> KTRY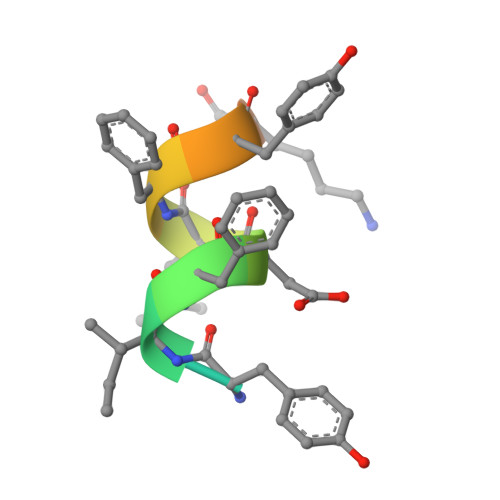IFDLFYKRKAY2-amino-6-propylpyrimidin-4(3H)-one | C7 H11 N3 O | 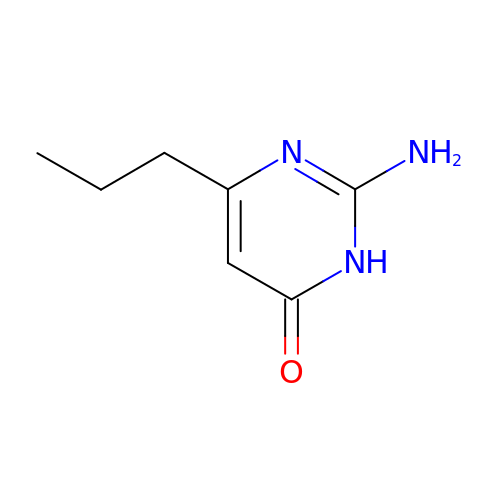FSYKBAWAYYELHH-UHFFFAOYSA-N> CLFS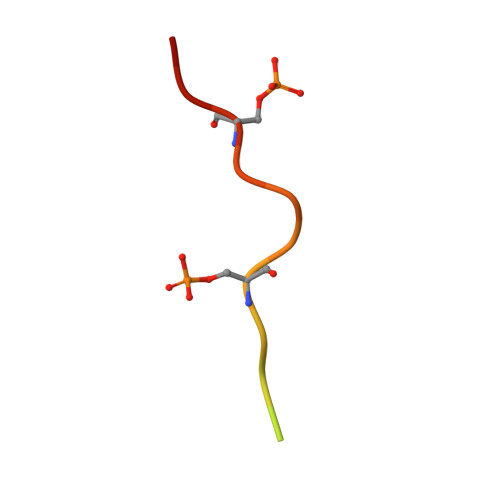GALSEGQFYSPPESFAG>[12x]MSKRKSYWNQGDKILLKNDVFMVDRYYDYYSNMGLNRFRWKNLPPGMESRHIEQALFNEGQAVFFKNTDPNEPYGFLCLPCAPSNGQNIYGDPVDFNGIGVNKYFTNLSPLNAVRILDNDNGLAPVRHIAYYTYLMSQIEMTINMNLDQQKFPIIIGATQKNKLSMENLYEKYSSFEPNILVDEKLAQALQEGKGFDALNTQAPYLLDK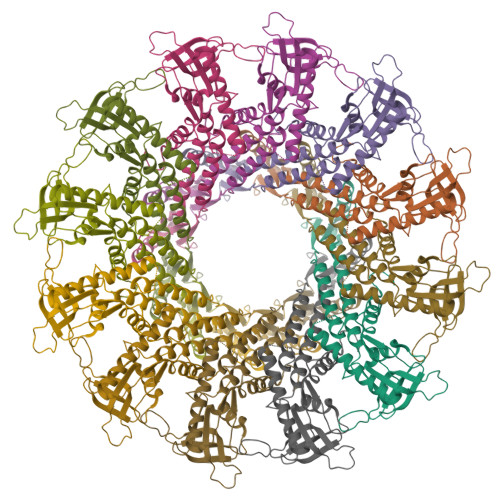LADFKKTCENELLTFLGINNTNNDKRERLLTDEVNANNSQITFVLEMAYKNRLDACKRINEMFGLNLEVEKVVNLLEVDMKGDVKNEGINGE Type III CRISPR-Cas systems employ multiprotein effector complexes bound to small CRISPR RNAs (crRNAs) to detect foreign RNA transcripts and elicit a complex immune response that leads to the destruction of invading RNA and DNA. The S. epidermidis effector complex, known as Cas10-Csm, consists of a crRNA and five Cas proteins: Cas10, Csm2, Csm3, Csm4 and Csm5. Target RNA binding activates single-stranded DNA (ssDNA) cleavage and cyclic oligoadenylates (cOAs) synthesis activities of Cas10-Csm. Type III CRISPR systems also possess the ability to degrade foreign RNA complementary to the crRNA (target RNA) via the Csm3/Cmr4 protein, and many complexes also have the ability to degrade single-stranded (ss) DNA via the HD nuclease domain of Cas10, comprising a complex multi-faceted interference response.

We performed cryo-EM reconstructions of the Type III-A Cas10-Csm effector complex from S. epidermidis bound to an intact, cognate target RNA and identified two oligomeric states, a 276 kDa complex and a 318 kDa complex. 3.1 Å density for the well-ordered 276 kDa complex allowed construction of atomic models for the Csm2, Csm3, Csm4 and Csm5 subunits within the complex along with the crRNA and target RNA. (E) The smaller complex consists of a 37 nt crRNA, two copies of Csm2 and three copies of Csm3. An additional difference between the complexes is present: Csm2 is well ordered in the 276 kDa complex but, while present, poorly ordered in the 318 kDa complex. Csm3 mediated target RNA cleavage was inhibitied during the incubation by the presence of EDTA, which chelates divalent metal ions required for the cleavage reaction. Comparison of the 276 kDa complex to previously published Cas10-Csm complexes of the same stoichiometry determined by cryo-EM indicates that we have captured a state of Cas10-Csm poised for catalysis. Csm2 is present in two copies in the 276 kDa complex, contacting target RNA in the vicinity of positions +13 to +24. The D32 residue of the RNase loop, which has been shown to be critical for target cleavage, is visible in the structure but is not coordinating a divalent metal ion, as it is expected to, because of the EDTA treatment of our sample prior to structural analysis. The 5’ nt of crRNA, position -8, is gripped by SeCsm4 via pi-stacking with residues F40 and H291. The β3’-loop and α1 appear to work in unison gripping the crRNA in the vicinity of nucleotides +17 to +21 in the 276 kDa complex.

> MTLATKVFKLSFKTPVHFGKKRLSDGEMTITADTLFSALFIETLQLGKDTDWLLNDLIISDTFPYENELYYLPKPLIKIDSKEEDNHKAFKKLKYVPVHHYNQYLNGELSAEDATDLNDIFNIGYFSLQTKVSLIAQETDSSADSEPYSVGTFTFEPEAGLYFIAKGSEETLDHLNNIMTALQYSGLGGKRNAGYGQFEYEIINNQQLSKLLNQNGKHSILLSTAMAKKEEIESALKEARYILTKRSGFVQSTNYSEMLVKKSDFYSFSSGSVFKNIFNGDIFNVGHNGKHPVYRYAKPLWLEV;>MILAKTKSGKTIDLTFAHEVVKSNVKNVKDRKGKEKQVLFNGLTTSKLRNLMEQVNRLYTIAFNSNEDQLNEEFIDELEYLKIKFYYEAGREKSVDEFLKKTLMFPIIDRVIKKESKKFFLDYCKYFEALVAYAKYYQKED[2x];>[3x]MYSKIKISGTIEVVTGLHIGGGGESSMIGAIDSPVVRDLQTKLPIIPGSSIKGKMRNLLAKHFGLKMKQESHNQDDERVLRLFGSSEKGNIQRARLQISDAFFSEKTKEHFAQNDIAYTETKFENTINRLTAVANPRQIERVTRGSEFDFVFIYNVDEESQVEDDFENIEKAIHLLENDYLGGGGTRGNGRIQFKDTNIETVVGEYDSTNLKIK;> MTIKNYEVVIKTLGPIHIGSGQVMKKQDYIYDFYNSKVYMINGNKLVKFLKRKNLLYTYQNFLRYPPKNPRENGLKDYLDAQNVKQSEWEAFVSYSEKVNQGKKYGNTRPKPLNDLHLMVRDGQNKVYLPGSSIKGAIKTTLVSKYNNEKNKDIYSKIKVSDSKPIDESNLAIYQKIDINKSEKSMPLYRECIDVNTEIKFKLTIEDEIYSINEIEQSIQDFYKNYYDKWLVGFKETKGGRRFALEGGIPDVLNQNILFLGAGTGFVSKTTHYQLKNRKQAKQDSFEILTKKFRGTYGKMKEIPSNVPVALKGTTNQSRHTSYQQGMCKVSFQELNNEVL> GSHMKNSVSVDLPGSMKVLVSKSSNADGKYDLIATVDALELSGTSDKNNGSGVLEGVKADASKVKLTISDDLGQTTLEVFKSDGSTLVSKKVTSKDKSSTYEKFNEKGELSEKKITRADKSSTYEKFNEKG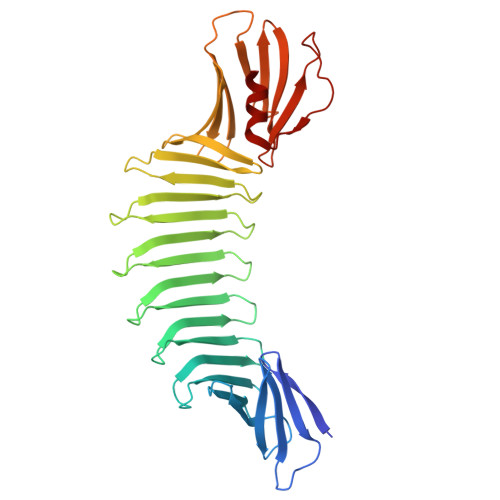ELSEKKITRADKSSTYEKFNEKGELSEKKITRADKSSTYEKFNEKGEVSEKIITRADGTRLEYTGIKSDGSGKAKEVLKGYVLEGTLTAEKTTLVVKEGTVTLSKNISKSGEVSVELNDTDSSAATKKTAAWNSGTSTLTITVNSKKTKDLVFTSSNTITVQQYDSNGTSLEGSAVEITKLDEIKNALK> MHHHHHHTTSVDPTSGPQASGTEQNRSSLDTAAARKLATTTKTVPQMQGISSRWLLRVLPWTQVNGGTYRVNRRLTHTLGDGQVEFVNTGAEVRVIPEELRELAPLRGFTDTPTLEALAGRFAQHEFAPGDVLAQQDQPADRIILIAHGKLDRLGTGKYGGETVQGQLAGGDHLGAAALLDGGAAWEHTVRAVTRVTALTLSRGDYEQVLGGSESLRAHVEAFRAALVPAQNKHGEAAIEVAAGHVGEPSLPGTFADYDLAPREYELSVAQTVLKIHSRVADLYNDPMNQMDQQLRLTVEALRERQEHEMINNREFGLLHNADLKQRIHTRSGPPTPDDLDELISRRRKTQVLLAHPRTIAAIGREWNARGIYPTGAELHGTDVRAWRGIPLLPCNKIPVTPEQTSSIIAMRLGEENQGVVGLHQTGIPDEYQPGLSVRFMGINDQAVIQYLVSAYYSAAVLVPDALGILEDVEIGH

Encapsulins are a prevalent protein‐based compartmentalization strategy in prokaryotes. Family 2, the most abundant class of encapsulins, is further subdivided into Family 2A and Family 2B based on the absence or presence, respectively, of a putative cyclic nucleotide binding domain (CBD) inserted into the E‐loop of the HK97 fold encapsulin shell protein. In this work, we report the characterization of a Family 2B two‐component encapsulin shell identified in Streptomyces lydicus (Sl). Through heterologous expression and purification studies, we show the differential assembly behavior of the two shell components – Sl‐Enc1 and Sl‐Enc2 – and demonstrate their ability to co‐assemble into mixed shells with variable shell composition.

In contrast, Sl‐Enc2 formed characteristic ca. 28 nm shells, consistent with other T = 1 Family 2B encapsulins. That is to say, the Sl‐Enc1 majority sample yielded a symmetry‐averaged Sl‐Enc1 shell map while the Sl‐Enc2 majority sample resulted in a symmetry‐averaged Sl‐Enc2 shell density. Sl‐Enc2 can assemble into complete shells by itself. Therefore, we used the symmetry‐averaged Sl‐Enc2 map to build a model for a complete homogeneous Sl‐Enc2 shell. The Sl‐Enc2 shell is 28 nm in diameter, consists of 60 identical protomers, and exhibits T = 1 icosahedral symmetry, similar to recently described Family 2B encapsulins. Overall, the homogeneous Sl‐Enc2 shell is similar to recently structurally characterized Family 2B encapsulins with externally displayed CBDs being positioned above all two‐fold pores. The two‐fold pores are large and elongated with dimensions of 14 by 60 Å and partially occluded by the CBDs. The absence of any resolvable N‐arms in the homogeneous Sl‐Enc2 shell contributes to the large dimensions of these pores. Two additional types of pores are present in the Sl‐Enc2 shell at the five‐ and three‐fold axes of symmetry with diameters of 6 and 3 Å, respectively. Symmetrical Sl‐Enc2 or mixed interactions never exhibited resolved N‐arms in our 3D classes.> GGSGPLKPEEHEDILNKLLDPELAQSERTEALQQLRVNYGSFVSEYNDLTK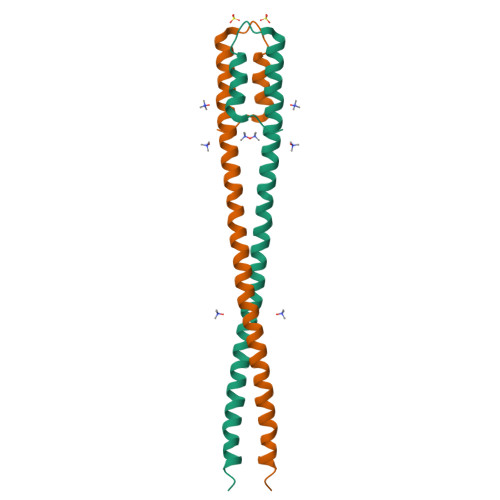RNNLLQAELEELRAVVEQTERSRKLAEQELIETSERVQLLHSQNTSLINQKKKMDADLSQLQTEVEEAVQECRNAEEKAEDLEKERDFYFGKLRNIELICQENEGENDPVLQRIVDILYATDEGFVIPD>[2x]XMEAAHSKSTEECLAYFGVSETTGLTPDQVKRHLEKYGHNELPAEEGKSLWELVIEQFEDLL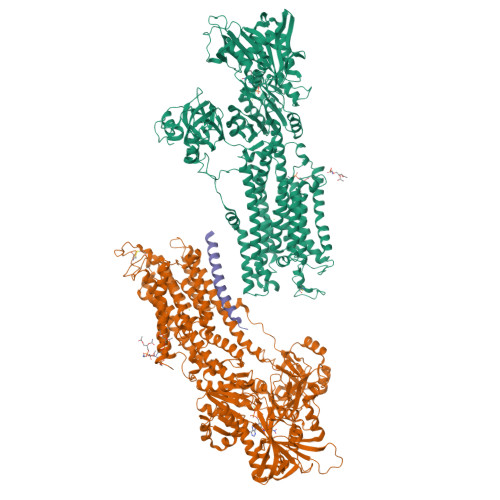VRILLLAACISFVLAWFEEGEETITAFVEPFVILLILIANAIVGVWQERNAENAIEALKEYEPEMGKVYRADRKSVQRIKARDIVPGDIVEVAVGDKVPADIRILSIKSTTLRVDQSILTGESVSVIKHTEPVPDPRAVNQDKKNMLFSGTNIAAGKALGIVATTGVSTEIGKIRDQMAATEQDKTPLQQKLDEFGEQLSKVISLICVAVWLINIGHFNDPVHGGSWIRGAIYYFKIAVALAVAAIPEGLPAVITTCLALGTRRMAKKNAIVRSLPSVETLGCTSVICSDKTGTLTTNQMSVCKMFIIDKVDGDFCSLNEFSITGSTYAPEGEVLKNDKPIRSGQFDGLVELATICALCNDSSLDFNETKGVYEKVGEATETALTTLVEKMNVFNTEVRNLSKVERANACNSVIRQLMKKEFTLEFSRDRKSMSVYCSPAKSSRAAVGNKMFVKGAPEGVIDRCNYVRVGTTRVPMTGPVKEKILSVIKEWGTGRDTLRCLALATRDTPPKREEMVLDDSSRFMEYETDLTFVGVVGMLDPPRKEVMGSIQLCRDAGIRVIMITGDNKGTAIAICRRIGIFGENEEVADRAYTGREFDDLPLAEQREACRRACCFARVEPSHKSKIVEYLQSYDEITAMTGDGVNDAPALKKAEIGIAMGSGTAVAKTASEMVLADDNFSTIVAAVEEGRAIYNNMKQFIRYLISSNVGEVVCIFLTAALGLPEALIPVQLLWVNLVTDGLPATALGFNPPDLDIMDRPPRSPKEPLISGWLFFRYMAIGGYVGAATVGAAAWWFMYAEDGPGVTYHQLTHFMQCTEDHPHFEGLDCEIFEAPEPMTMALSVLVTIEMCNALNSLSENQSLMRMPPWVNIWLLGSICLSMSLHFLILYVDPLPMIFKLKALDLTQWLMVLKISLPVIGLDEILKFIARNYLEG;> MERSTRELCLNFTVVLITVILIWLLVRSYQY>MSNEIPKPVAPAPDILRCAYAELVVTDLAKSRNFY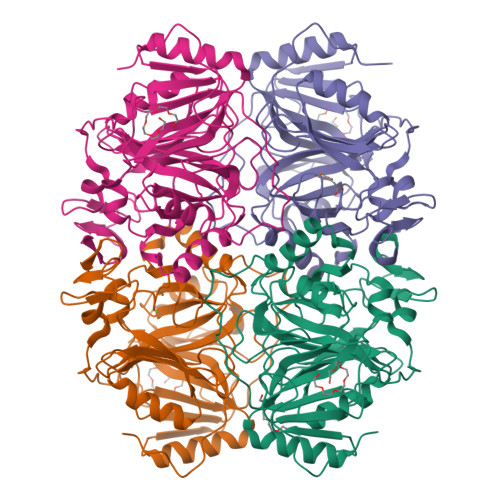VDVLGLHVSYEDENQIYLRSFEEFIHHNLVLTKGPVAALKAMAFRVRTPEDVDKAEAYYQELGCRTERRKDGFVKGIGDALRVEDPLGFPYEFFFETTHVERLHMRYDLYSAGELVRLDHFNQVTPDVPRGRKYLEDLGFRVTEDIQDDEGTTYAAWMHRKGTVQDTALTGGNGPRLHHVAFSTHEKHNIIQICDKMGALRISDRIERGPGRHGVSNAFYLYILDPDNHRIEIYTQDYYTGDPDNPTITWNVHDNQRRDWWGNPVVPSWYTEASKVLDLDGNVQEIIERTDDSELEVTIGADGFSFTRAGDEDGSYHGQASKGFKLGNQL[4x]> GIDPFTTRPSSDLTAFREHFAKAKHIAIITGAGVSAESGVPTFRGPGGFWRKWQAQDLATPEAFSRDPSLVWEFYHYRREVMRSKMPNPAHLAIAECEARLGQQGRSVVIITQNIDELHHRAGSKHVYEIHGSLFKTRCMSCGEVKANHKSPICPALDGKGAPDPNTKEARIPVELLPRCERKSCNGLLRPHVVWFGETLDSDILTAVERELEKCDLCLV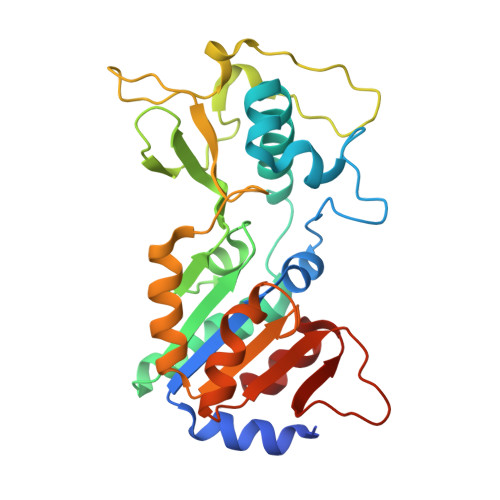VGTSSIVYPAAMFAPQVASRGVPVAEFNMECTPATQRFKYHFEGPCGSTLPPALE>MDTILLTGLFAAFFTTFAFAPQSIKTIRTRNTEGISV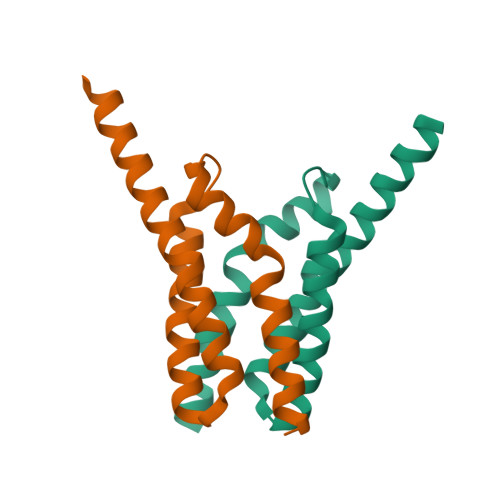VMYIMFLTGVISWIAYGIMRSDFAVLIANIVTLFLAAPVLVITLINRRKKHVLESSGENLYFQ[4x]> TFDTPKHRCGSEITNSYMDLC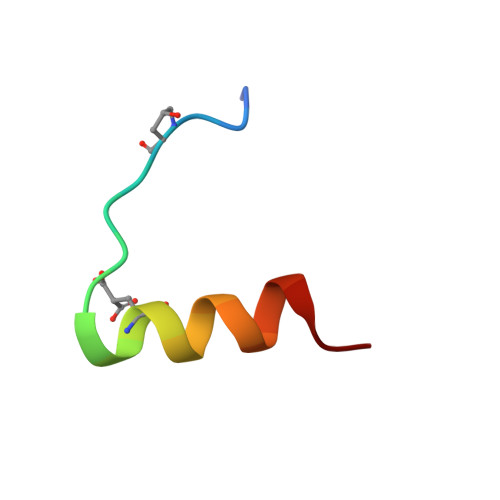YR>MG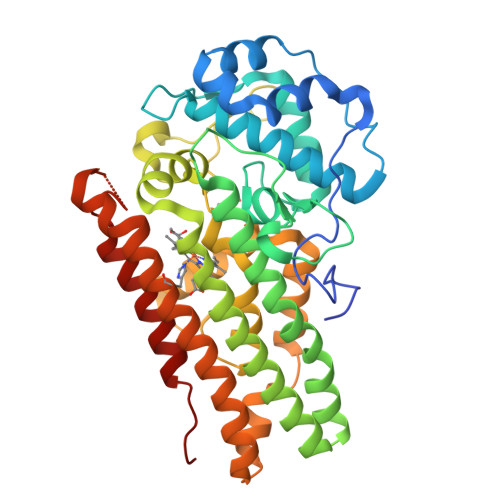SSHHHHHHSSGSAAYHIDEEVGFALPNPQENLPDFYNDWMFIAKHLPDLIESGQLRERVEKLNMLSIDHLTDHKSQRLARLVLGCITMAYVWGKGHGDVRKVLPRNIAVPYCQLSAALELPPILVYADCVLANWKKKDPNKPLTYENMDVLFSFRDGDCSKGFFLVSLLVEIAAASAIKVIPTVFKAMQMQERDTLLKALLEIASCLEKALQVFHQIHDHVNPKAFFSVLRIYLSGWKGNPQLSDGLVYEGFWEDPKEFAGGSAGQSSVFQCFDVLLGIQQTAGGGHAAQFLQDMRRYMPPAHRNFLCSLESNPSVREFVLSKGDAGLREAYDACVKALVSLRSYHLQIVTKYILIPASQQPKENKTSEDPSKLEAKGTGGTDLMNFLKTVRSTTEKSLLKEG[4x]3-[(4,6-dipyridin-4-yl-1,3,5-triazin-2-yl)amino]-4-methyl-~{N}-[3-(trifluoromethyl)phenyl]benzamide | C28 H20 F3 N7 O | 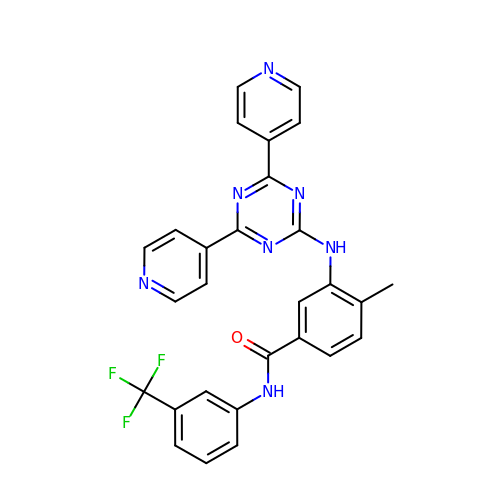QRGMMQTYOVICBC-UHFFFAOYSA-N> GNNVVVLGTQWGDEGKGKIVDLLTERAKYVVRYQGGHNAGHTLVINGEKTVLHLIPSGILRENVTSIIGNGVVLSPAALMKEMKELEDRGIPVRERLLLSEACPLILDYHVALDNAREKARGAKAIGTTGRGIGPAYEDKVARRGLRVGDLFDKETFAEKLKEVMEYHNFQLVNYYKAEAVDYQKVLDDTMAVADILTSMVVDVSDLLDQARQRGDFVMFEGAQGTLLDIDHGTYPYVTSSNTTAGGVATGSGLGPRYVDYVLGILKAYSTRVGAGPF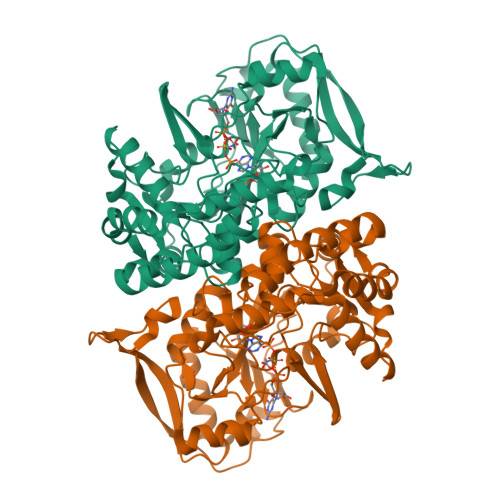PTELFDETGEFLCKQGNEFGATTGRRRRTGWLDTVAVRRAVQLNSLSGFCLTKLDVLDGLKEVKLCVAYRMPDGREVTTTPLAADDWKGVEPIYETMPGWSESTFGVKDRSGLPQAALNYIKRIEELTGVPIDIISTGPDRTETMILRDPFDA>[8x]MNFEGKIALVTGASRGIGRAIAETLAARGAKVIGTATSENGAQAISDYLGANGKG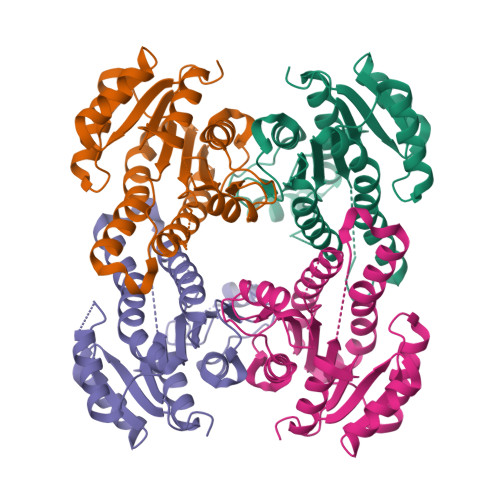LMLNVTDPASIESVLEKIRAEFGEVDILVNNAGITRDNLLMRMKDEEWNDIIETNLSSVFRLSKAVMRAMMKKRHGRIITIGSVVGTMGNGGQANYAAAKAGLIGFSKSLAREVASRGITVNVVAPGFIETDMTRALSDDQRAGILAQVPAGRLGGAQEIANAVAFLASDEAAYITGETLHVNGGMYMV>[2x]QLTFQTSSPAHLTMPYVMPGD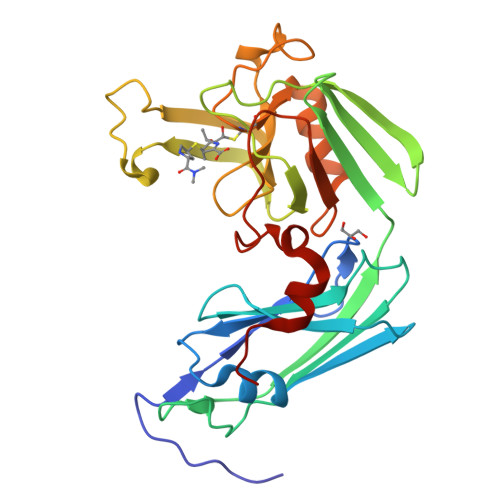GEVVGVGEPVAIRFDENIADRGAAEKAIKITTNPPVEGAFYWLNNREVRWRPEHFWKPGTAVDVAVNTYGVDLGEGMFGEDNVQTHFTIGDEVIATADDNTKILTVRVNGEVVKSMPTSMGKDSTPTANGIYIVGSRYKHIIMDSSTYGVPVNSPNGYRTDVDWATQISYSGVFVHSAPWSVGAQGHTNTSHGCLNVSPSNAQWFYDHVKRGDIVEVVNTVGGTLPGIDGLGDWNIPWDQWRAGNAKA>[2x]MGSSHHHHHHSSGPQQGLRQHANVVWDTPSRNSSESMPCGGGDIGMNIWVEE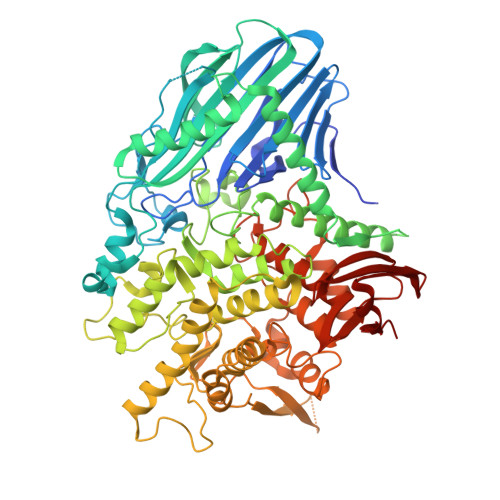GDILFYLSRSGTFDENNCQLKQGRFRLRLSPNPFEDAKDFRQELKLIDGYVEISAEGTQVQLWADVFHPVVHIEVINDRPLQAEIFYENWRYQDRLIRKGEGQQCSYKWAPPKGTMTHADFISLENSSEKDSKRLLFYHRNAEETVFDVAVAQQGMNEVKSQMMNPLKNLTFGGYLSGENLEYIGTSDSVYAGTDYRAWGFRSLKASKKHHFSVVLHTEQTETVTQWEQGLKTAWQRIAPQGKISSKVVSQDKKQTRLWWNAFWQRSFIETIGETENKENSKVEKETGNKEKSDAKDALKEITRNYTLFRYMLGCNAYGSVPTKFNGGLFTFDPCHIDEKQAFTPDYRKWGGGTMTAQNQRLVYWPMLKSGDFDMMPSQFNFYNRMLKNAELRSHVYWQHEGACFCEQIENFGLPNPAEYGFKRPAWFDKGLEYNAWLEYEWDTILEFCQMILETKNYAGADITPYLPLIESSLTFFDEHYRLLASRRGRKALDGDGHLILFPGSACETYKMTNNASSTIAALRTVLETYIKVCNNEKWQKMLETIPPVPLRYIEVKDSLNLQASTMTPAWKQTISPAKSWERINNIETPQLYPVFPWRIYGVGKENLEIARDTYFYDPDALKFRSHTGWKQDNIWAACLGLTEEAKSLSLAKLSDGPHRFPAFWGPGYDWTPDHNWGGSGMIGLQEMLLQTNGTQILLFPAWPKEWNVHFKLHAPGNTTVEATLKDGKVTILKVSPESRKKDIVIMIEK DICYCLOPENTYL PHOSPHORAMIDATE | C10 H20 N 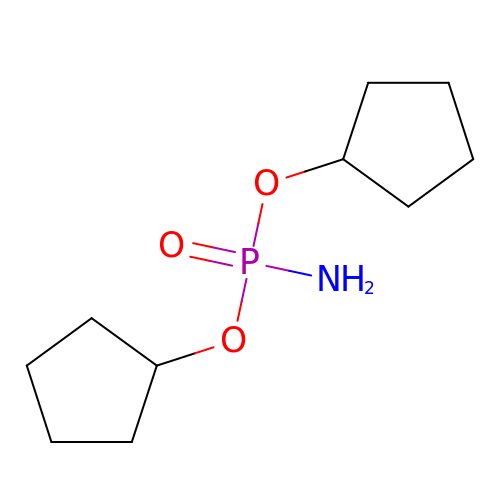O3 P | BDYGAPLPLXNVSE-UHFFFAOYSA-N> GAMDPMIIR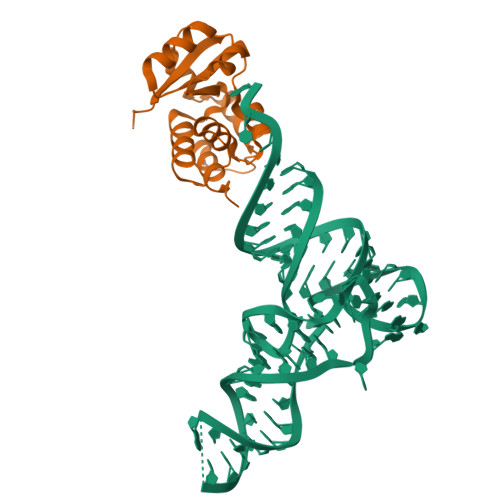GIRGARINNEIFNLGLKFQILNADVVATKKHVLHAINQAKTKKPIAKSFWMEILVRASGQRQIHEAIKIIGAKDGNVCLICEDEETFRKIYELIGGEIDDSVLEINEDKERLIREIFKIRGFGNVVERVLEKIALIELKKE5'-O-(benzylcarbamoyl)guanosine | 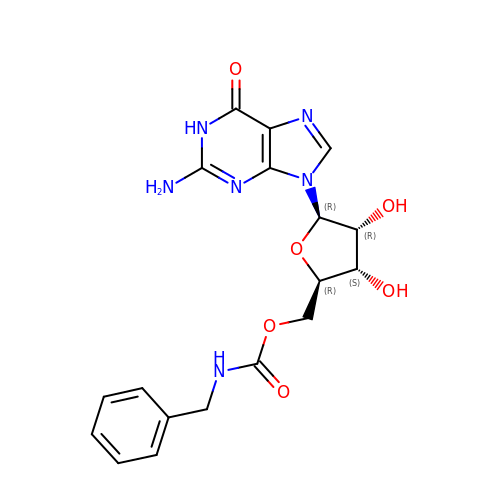C18 H20 N6 O6 | LCCRNJDOCQAPJZ-XNIJJKJLSA-N> MIDLREDTWTLQLYAQRYKGLSPKNSRELQLRMEYDPLKPNLPTSGEEQNSKPEWLNTPPCLIPESESLDKAKGALVGLAIGDAIGTTLEFLPRDKLHVNDMVGGGPFRLQPGEWTDDTSMALCLAESYISAGRLDITLFREKLVRWYRHGENSSNGRCFDIGNTTRNALEQYLKHGASWFGNTEPETAGNAAIIRQAPTSIFRRKSLQRTFADSDSQSMATHCAPESMASC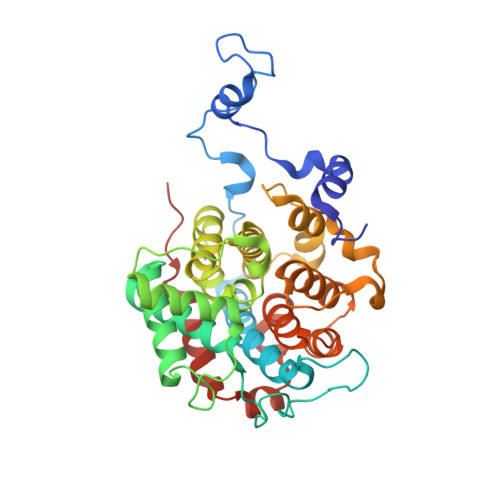QFLGFILNYLINGSSREKAFSPHVMPLPVRVLLINAGEYKEKKRDEIRSSGYVIDTLEAAMWAVWNTDNFHDAILLAANLGDDADSVAATTGQIAGALYGYSNIPKPWLDKLVQQERISNLAEQLFYMAPEEDF>[2x]TRKAVIGYYFIPTNQINNYTETDTSVVPFPVSNITPAKAKQLTHINFSFLDINSNLECAWDPATNDAKARDVVNRLTALKAHNPSLRIMFSIGGWYYSNDLGVSHANYVNAVKTPASRAKFAQSCVRIMKDYGFDGVDIDWEYPQAAEVDGFIAALQEIRTLLNQQTITDGRQALPYQLTIAGAGGAFFLSRYYSKLAQIVAPLDYINLMTYDLAGPWEKVTNHQAALFGDAAGPTFYNALREANLGWSWEELTRAFPSPFSLTVDAAVQQHLMMEGVPSAKIVMGVPFYGRAFKGVSGGNGGQYSSHSTPGEDPYPSTDYWLVGCEECVRDKDPRIASYRQLEQMLQGNYGYQRLWNDKTKTPYLYHAQNGLFVTYDDAESFKYKAKYIKQQQLGGVMFWHLGQDNRNGDLLAALDRYFNAADYDDSQLDMGTGLRYTGVGPGNLPIMTAPAYVPGTTYAQGALVSYQGYVWQTKWGYITSAPGSDSAWLKVGRV

Glycoside hydrolase family 18 (GH18) chitinases (EC 3.2.1.14) catalyse the degradation of chitin, a homopolymer of β-(1,4)-linked N-acetylglucosamine, which play important roles in various life processes. For instance, the well-studied bacterium Serratia marcescens produces several GH18 chitinases to efficiently degrade chitin for nutrition. Because of the extensive roles of GH18 chitinases, inhibitors targeting these enzymes have potential applications as therapeutic agents and agrochemicals. In this study, we used SmChiB, a model GH18 chitinase from the bacterium S. marcescens, to improve inhibitory activity of berberine.

In this study, we found berberine was also a competitive inhibitor against SmChiB, a well-studied GH18 chitinase, with a Ki value of 11.79 μΜ. The crystal structure of the SmChiB-berberine complex was obtained by soaking and was resolved to a resolution of 1.94 Å. The crystal complex structure clearly revealed the location of berberine in the active pocket of SmChiB. Berberine occupied the active pocket across the sugar-binding subsites +1 and +2 which was characterised by the aromatic Trp97 and Trp220, respectively. The conjugate tetracycle plane of berberine was sandwiched by Trp97 and Trp220 to form π-π stacking interactions within distance of 4.2 and 4.3 Å respectively. This observation was consistent with our previous work that berberine inhibited GH18 chitinases mainly via π-π stacking interactions between the tetracycle plane and the aromatic residues in the binding pockets. Moreover, an unoccupied hydrophobic cavity formed by residues Phe190, Phe191, Leu216, Phe239, and Leu265 was identified. This space provides a favourable opportunity for the optimisation of berberine at its 9-O-position or 10-O-position. The binding modes of 4a-4c against SmChiB were nearly identical to that of berberine. As a result, the berberine analogues were able to form additional interactions such as hydrogen bonds and stacking interactions with surrounding residues of SmChiB, which may account for their increased inhibitory activities.In the fourth step in this pathway, UDP-2,3-diacylglucosamine is hydrolyzed to 2,3-diacylglucosamine-1-phosphate (also called lipid X) and UMP. This step is catalyzed by the specific pyrophosphatase LpxH in 70% of gram-negative bacteria, including E. coli and Pseudomonas aeruginosa, and by LpxI in the remaining 30%345. LpxH shares sequence similarity with metallophosphoesterases and requires Mn2+ ions for phosphatase activity. PaLpxH consists of two domains: a catalytic domain homologous to metallophosphoesterases (MPEs) and a helical insertion domain (HI domain) inserted in the middle of the catalytic domain.

PaLpxH was crystallized in the presence of Mn2+ ions, which are required for enzymatic activity. Two PaLpxH molecules were present in the asymmetric unit of the P21 crystal, and all 239 amino acid residues were unambiguously determined for both molecules. Furthermore, the high-resolution electron density (1.65 Å) clearly identified a stoichiometrically bound product molecule (lipid X, 2,3-diacylglucosamine-1-phosphate) and two Mn2+ ions in each PaLpxH molecule. The lipid X molecule was likely captured in E. coli cells because no substrate molecule (UDP-2,3-diacylglucosamine) or product molecule (lipid X) was added during purification or crystallization. At the boundary between the catalytic and HI domains, invariant residues and two Mn2+ ions form a dinuclear metal center. Lipid X is positioned in a crevice between the catalytic and HI domains, with the phosphate group facing the dinuclear metal center and two acyl chains buried in the hydrophobic cavity. Six ligands [Asp8, His10, Asp41 (bridging two Mn2+ ions), His197, and two hydroxide ions (designated as W1 and W2)] are octahedrally coordinated with Mn1. In contrast, five ligands provide an incomplete octahedral coordination with Mn2: Asp41, Asn79, His114, His195, and W2 (bridging two Mn2+ ions). In the EP complex, the phosphate group of lipid X (corresponding to the beta phosphate moiety of UDP-2,3-diacylglucosamine) is strongly bound to Arg80 through a bidentate salt bridge. W1 is positioned close enough to attack the alpha phosphate of the substrate in the ES complex, as deduced from the structure of the EP complex.

>MSVLFISDLHLEAERPDITRAFLSFLDERARRAEALYILGDFFEAWIGDDGMDAFQRSIAQSLRQVADGGTRIYLMHGNRDFLIGKAFCREAGCTLLPDPSVIDLYGEPVLLMHGDSLCTRDEAYMRLRRWLRNPLTLWVLRHLPLATRHKLARKLRKESRAQTRMKAVDIIDVTPEEVPRVMRGHGVRTLIHGHTHRPAEHPLDIDGQPARRIVLGDWDRQGWALEIDANGHRQAPFPLLEHHHHHH[2x]>MAQSSNSTHEPLEVLKEETVNRHRAIVSVMEELEAVDWYDQRVDASTDPELTAILAHNRDEEKEHAAMTLEWLRRNDAKWAEHLRTYLFT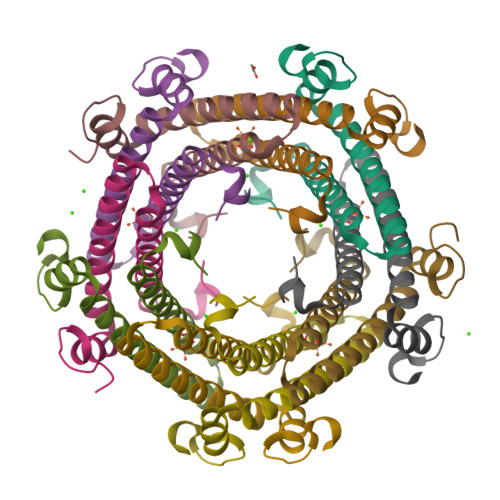EGPITAANSSSVDKLAAALEHHHHHH[30x]>VIQNSLNDKIVTISCKADTNLFFYQVAGNVSLFQQTRNYLERWRLIYDSNKAAYKIKSMDIHNTNLVLTWNAPTHNISTQQDSNADNQYWLLLKDIGNNSFIIASYKNPNLVLYADTVARNLKLSTLNNSNYIKFIIEDYIISDLNNFTCKISPILDLNKVVQQVDVTNLNVNLYTWDYGRNQKWTIRYNEEKAAYQFFNTILSNGVLTWIFSNGNTVRVSSSNDQNNDAQYWLINPVSDTDETYTITNLRDTTKALDLYGG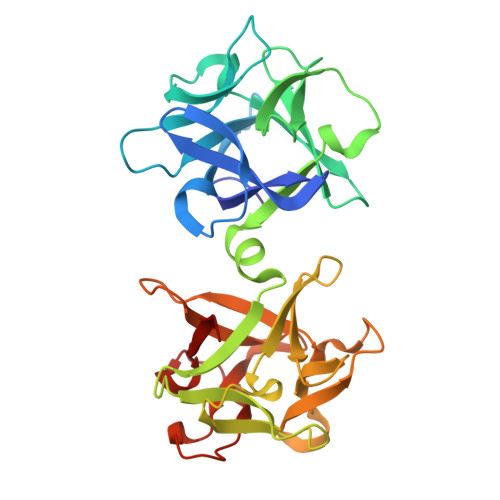QTANGTAIQVFNYHGDDNQKWNIRNP[2x]>[4x]MAEAGITGTWYNQL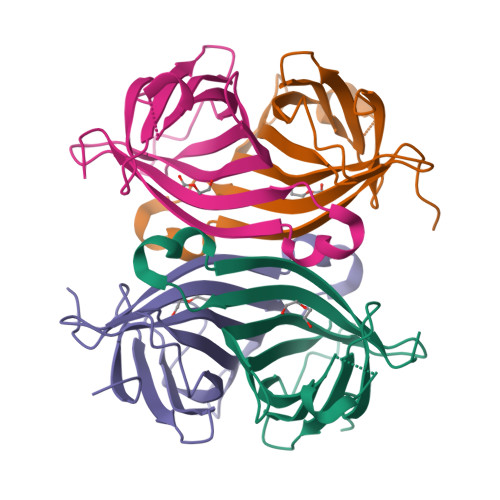GSTFIVTAGADGALTGTYESAVGNAESRYVLTGRYDSAPATDGSGTALGWTVAWKNNYRNAHSATTWSGQYVGGAEARINTQWLXTSGTTEANAWKSTLVGHDTFTKVKPSAASLEHHHHHH> MIELPDAISDGEVRKLVENEFWPEFVRRREKLDRIAQWARGEQPDYLIQNANREKRALLKLAKTPWLGLVVTHFTQALFVDGYRAEGSKENAKGPWQTWNANKMQSKQIAIHRAALTYGYSYARVLPGVALDGANQAEIHGVSPRRLLALYEDQINDEYPKYALELANNGKTVRLYTDTDYYELRMPSPGNFPNEQVIKKVHHGVGVCPFVRYVNMMDLDGFTMGEVEYLVPVASKIDKTDYDRLLAQHYNSW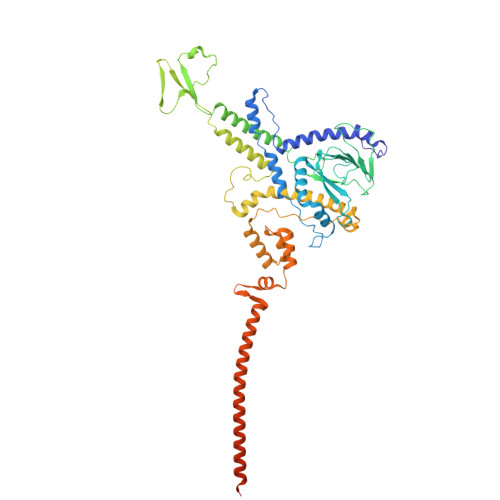KVKVATGIDDLSEDATPEEQQRAKLILAQDDILMHGNHEAKFYTLPETSLDGFIAAHTQDVEILANNAQVPVWILNGQLANLSADALTAATKGTIQKLYERQVTFGAAHNQVLRLAAHVEGDTEGARDFTASVSWQDTSVRSLAQAVDAYGKAATMLGMPKEFLWGLIPGITKTDVEAMRQHFNDDDEMTQMLLWWTPNGPGGEFAAEIEVDSQTQIIEAQGDVQKDLQDAQAKAQADLAKQNAAAQQRQAVAVAKATPAASKAPSTSKAASKRTPKKQGGVSGNDPASRAA> SMSEQSICQARAAVMVYDDANKKWVPAGGSTGFSRVHIYHHTGNNTFRVVGRKI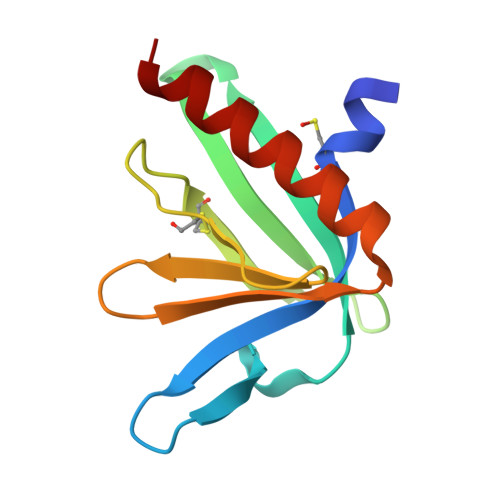QDHQVVINCAIPKGLKYNQATQTFHQWRDARQVYGLNFGSKEDANVFASAMMHALEVLNS>[9x]FTLVELIVVIIIIAIIAAVAIPAITSFQDNARKSRIQSEHRELVSAIQSYIGAQDDPTNPSEITLAKLAPYMSKNAKNEDGIVNSLAKDKSGNSSTSAPGSAHQIDTTNHKLISTFTPSNGGQATVLTYDWSANGVNSN

Type 4 pili (T4P) are important virulence factors, which belong to a superfamily of nanomachines ubiquitous in prokaryotes, called type 4 filaments (T4F). T4F are defined as helical polymers of type 4 pilins. S. sanguinis T4P have been characterised in depth, revealing that they are heteropolymers of two major pilins (PilE1, PilE2)—which is unusual—and three minor pilins (PilA, PilB, PilC). Our 3.7 Å resolution cryo-EM structure of S. sanguinis heteropolymeric T4P and the resulting full atomic model including all minor pilins highlight universal features of bacterial T4F and have widespread implications in understanding T4F biology.

After 3D refinement and local refinement on the central portion along the filament axis (150 Å long), we generated a final density map at 3.7 Å resolution, as estimated by gold-standard Fourier shell correlation (FSC). The resolution, which is close to 3.3 Å in the central portion of the filament, decreases to 4.3 Å towards the edges, especially towards both ends. This made it impossible to precisely calculate the helical symmetry operators for the filament, which could nevertheless be estimated at 11 Å in rise and 93° in twist angle. As PilE1 and PilE2, which could not be distinguished within the final density map, share high sequence identity, we arbitrarily chose PilE1 to produce an atomic model of S. sanguinis T4P. In our atomic model, the pilin subunits display a canonical lollipop structure in which the α1N portion of a 52 residues-long α1 helix protrudes from a globular head. In the globular head, α1C is packed against a three-strand β-sheet, which is flanked at its N- and C-termini by two regions with limited secondary structure elements, a large αβ-loop and a short CT tail, respectively. Critically, as in other structures of bacterial T4F11, a portion of α1N is melted, the extent of which varies slightly between Ile16 and Gln28 in the different chains. The superposition of the structures of the complete pilins that we were able to resolve, shows that the α1N up to the end of the melted region are intrinsically flexible, emanating at different angles from the globular heads, which in contrast remain almost unchanged, aligning with 1.3 Å root-mean-square deviation (RMSD) globally. The filaments are right-handed with four pilins per turn, displaying approx. 11 Å rise and 93° twist between consecutive subunits within the 1-start helix. Perhaps the most unusual interaction is within the right-handed 1-start helix, where the CT tail in PilE1 (mostly negatively charged) engages the next pilin αβ-loop (mostly positively charged) through electrostatic interactions. At the level of the left-handed 3-start, the melted region in subunit S is held in a groove between α1N of subunit S+3, and α1C of subunit S−3.Flavoxate | C24 H25 N O4 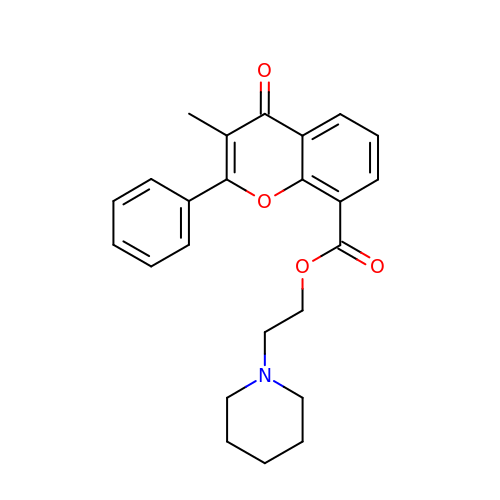| SPIUTQOUKAMGCX-UHFFFAOYSA-N> SVALVPHVGMGLETRTE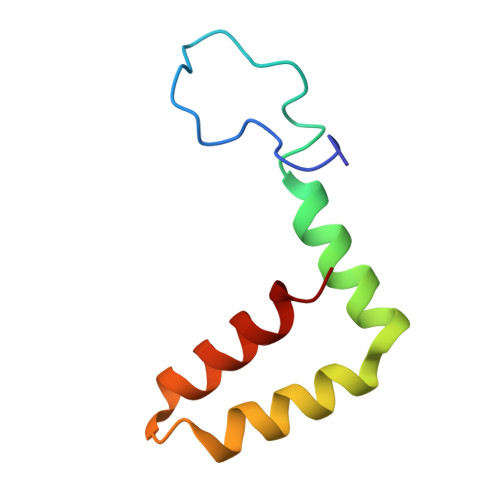TWMSSEGAWKHAQRIETWILRHPGFTIMAAILAYTIGTTHFQRALIFILLTAVAP>[2x]MISNDIAIDLGTANTLIYQKGKGIVLNEPSVVALRNVGGRKVVHAVGIEAKQMLGRTPGHMEAIRPMRDGVIADFEVAEEMIKYFIRKVHNRKG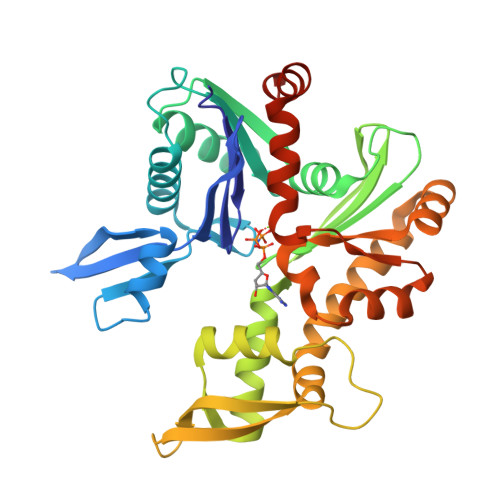SGNPKVIVCVPSGATAVERRAINDSCLNAGARRVGLIDEPMAAAIGAGLPIHEPTGSMVVDIGGGTTEVAVLSLSGIVYSRSVRVGGDKMDEAIISYMRRHHNLLIGETTAERIKKEIGTARAPADGEGLSIDVKGRDLMQGVPREVRISEKQAADALAEPVGQIVEAVKVALEATPPELADDIADKGIMLTGGGALLRGLDAEIRDHTGLPVTVADDPLSCVALGCGKVLEHPKWMKGVLESTLAGSHHHHHH>[2x]MPGETITLQVGQCGNQVGLQYWQQLATEHGIQSDGSSTPYPKDINDLQLQELNNSGSSPQSYPQQTKPNGKYRNDHPELFFTLSDSNTYTPRSILIDMEPSVIAKSTSALPMFNPRNVHLSNQGNGAANNWINGYKYGTEEEETLLNLIDREVDKCDNLSNFQLFHSVAGGTGSGVGSKMLEVISDRYGHKKLLNTFSIFPSNEDTSDVVVQPYNTILTLKRLIDYSDATFVFHNDSLNRIENILFNNNSNIQHDDNDLFLGANKLIALVSASVSNPLRFPGYMYSSMESIVSNLIPTPDLKFLTSSIAPFSTQKHNYLNEYDMLLELSNDRYKTNRVGGDTSYISMLNYLIGYNLDQREIRKGILKSQQRISFVPWVARSVLVVHGKKSPYLKNTNLEGIQVTNNTSMIDVFTKILKQFDLLIKRKAYLNRYYSSVEEENEVMEMFNESRESVKSIIDEYKACKEITYLDDDDEDDLEDGDGGGGGNGNGYNNIDDADMGI;> MNTFSSPPNVIREYNDSTYQSPLNSQFHQSPFLQTQSPDYVSLREEEDDNNDKNLDIMSSCIVDSVIYKSQKIAGPLLSQISNLNIQQALIIRELLFTLLGHEGHYIQYSKRYDPTSQISRIEGPDYKIAKNLDISLKVITKKLVKFGKFYSGLKSFIQVFDNNKFGKIVQKFCSEVRKFLSSYQQVLINVEHEFKFNKNFNLNMLDSLLHQEISNEMTHLYQIGIEISRITEERQKMSQAEIMGNFEPTTLANTSMNGINSEPNLYYGKFDCCKGGLLLQ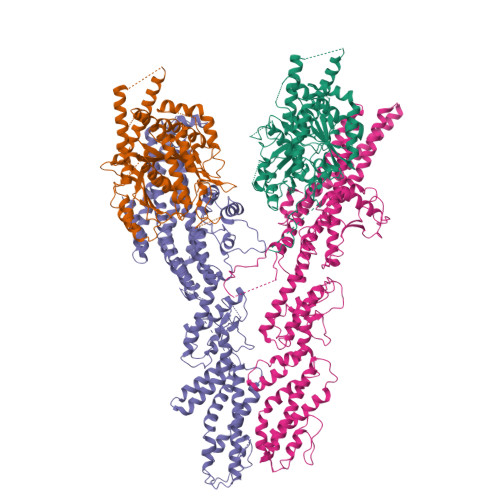VIQERMVYYKGDPTSLDFLTQLFDIVSSDYIGMLNQWLLEGVINDPFDEFMIREKRVPDSFMEIFQSKSEYYWNELFLIKIDGLLNQFQNSTIQSKILNTGKYLNIFKRCTGLHNFESLKEKLTTITSLAAPDLELKIDEFYHRANKMLMKLLFDGYNFPSVVNIFQRLFLFADSFQIDNFIDSTFSELKRGKLKISVSRLQKQYDDIFKEKIENKVGVRPSVYDVLKKNQKLSVTSESLYKVVEELMEKNSDYLISDNNLRGIFHRVASLRDDSRLTISSTADSATENVKDEPTITSVDLTIPLPFPLNLVLNQQLSYQYEIMFKLLINIKFISKYNSSNWQEMNYSKIWTNSHFNSSVKKWILRCRVLHSRICSFIHELENYIVHDVIEHNFEEIKNLIHTTATNLATSELGSDINDEGDNIFNGSLIRGTFNNNSIFDSKVHKHRTTTYVEGISTVEQLIQKFLDYSSTLLNDSLLTREESLRQLRKMLDFIFHFNNYIVQVKKVLVLLNHELFNEYSKEFPTKFEKPMDQESIDKRFANLSDTFLMQYEKFGENLVTFLATIKQVGERENQGLLELSNRLELCFPE;> MALNKVQLIKLYSNRLVKSLVPVEFGEAFIQSIINDLQTTLLNTSSEEQNLSIIINKLKMQFLSNNLKNEWVEFQNIVNSLSKFKSLDQICNYLAFLDALRDEKPEDILSTSTASLSPGKQNLMINTVNTALTLSQLIEPYYDTLSEQTILTYLPYTMLGSDSKIFTFSNNYTRLEIPKDINNSFSSLLREVFEFAILYKQLAIVVDRYKGTLVSAIKTAYIAILEAQLNKYVNDINNIFNNKPNSILVVYNSIFPWISILRFLYRVSNRLNRLDGYEFLTFIYSFTNHGDPKIRGIAVTAFTEVVKPYYNIVEHWIVKGELIDNNNEFFIIFDQEQNEFNSIIKLLPKKIPAFIKSSDKIFQIGKTLIFLNKYCRELKWVNQYNVKYSAILFNNHQGLASMTTNEMIKLIDSQYNEILTFLTQIIQGNNKLFTHVYNFKRFYFMETNDFIDAIMVKGKDVFNESSVNISSTYLRKVLQDAIQISSVKNFEYVDRLDSRVLNPQHGNLGWESFTIEYKIDDLPMSYLFEGHQHLQYLKMFHFLWKLRQLNNLLNWHFEMFNELNHNVVTKLSSRNRRPLAKSLSIITSIRFHFTQFLNELIAYLSYDVIEENFQQHIVRKLFYNKNDQDLLLNKSFMNLSEIDPNNDLPKFNVNLLTIDELVELHGTYIDSIINSSLLNEKLKGNETNISYIDQIFNILQTIFNFINTSQEFYSLVVTFGLLVRSDSNANKIELEQDQEDLEFQLHKIKRKIYKDIYQHDYKRQLNDLKNDLNRDYNLKDLSKLL> MSDSVILRSIKKFGEENDGFESDKSYNNDKKSRLQDEKKGDGVRVGFFQLFRFSSSTDIWLMFVGSLCAFLHGIAQPGVLLIFGTMTDVFIDYDVELQELQIPGKACVNNTIVWTNSSLNQNMTNGTRCGLLNIESEMIKFASYYAGIAVAVLITGYIQICFWVIAAARQIQKMRKFYFRRIMRMEIGWFDCNSVGELNTRFSDDINKINDAIADQMALFIQRMTSTICGFLLGFFRGWKLTLVIISVSPLIGIGAATIGLSVSKFTDYELKAYAKAGVVADEVISSMRTVAAFGGEKREVERYEKNLVFAQRWGIRKGIVMGFFTGFVWCLIFLCYALAFWYGSTLVLDEGEYTPGTLVQIFLSVIVGALNLGNASPCLEAFATGRAAATSIFETIDRKPIIDCMSEDGYKLDRIKGEIEFHNVTFHYPSRPEVKILNDLNMVIKPGEMTALVGPSGAGKSTALQLIQRFYDPCEGMVTVDGHDIRSLNIQWLRDQIGIVEQEPVLFSTTIAENIRYGREDATMEDIVQAAKEANAYNFIMDLPQQFDTLVGEGGGQMSGGQKQRVAIARALIRNPKILLLDMATSALDNESEAMVQEVLSKIQHGHTIISVAHRLSTVRAADTIIGFEHGTAVERGTHEELLERKGVYFTLVTLQSQGNQALNEEDIKDATEDDMLARTFSRGSYQDSLRASIRQRSKSQLSYLVHEPPLAVVDHKSTYEEDRKDKDIPVQEEVEPAPVRRILKFSAPEWPYMLVGSVGAAVNGTVTPLYAFLFSQILGTFSIPDKEEQRSQINGVCLLFVAMGCVSLFTQFLQGYAFAKSGELLTKRLRKFGFRAMLGQDIAWFDDLRNSPGALTTRLATDASQVQGAAGSQIGMIVNSFTNVTVAMIIAFSFSWKLSLVILCFFPFLALSGATQTRMLTGFASRDKQALEMVGQITNEALSNIRTVAGIGKERRFIEALETELEKPFKTAIQKANIYGFCFAFAQCIMFIANSASYRYGGYLISNEGLHFSYVFRVISAVVLSATALGRAFSYTPSYAKAKISAARFFQLLDRQPPISVYNTAGEKWDNFQGKIDFVDCKFTYPSRPDSQVLNGLSVSISPGQTLAFVGSSGCGKSTSIQLLERFYDPDQGKVMIDGHDSKKVNVQFLRSNIGIVSQEPVLFACSIMDNIKYGDNTKEIPMERVIAAAKQAQLHDFVMSLPEKYETNVGSQGSQLSRGEKQRIAIARAIVRDPKILLLDQATSALDTESEKTVQVALDKAREGRTCIVIAHRLSTIQNADIIAVMAQGVVIEKGTHEELMAQKGAYYKLVTTGSPIS

BSEP (ABCB11) is an ATP-binding cassette transporter that is expressed in hepatocytes and extrudes bile salts into the canaliculi of the liver. BSEP dysfunction, caused by mutations or induced by drugs, is frequently associated with severe cholestatic liver disease. BSEP has two transmembrane domains (TMDs), each composed of six TM helices, and two nucleotide-binding domains (NBDs). The NBDs of BSEP are predicted to form one functional nucleotide-binding site (NBS2, consisting of Walker-A and Walker-B motifs of NBD2 and the signature motif of NBD1), and one degenerate nucleotide-binding site (NBS1, consisting of Walker-A and Walker-B motifs of NBD1 and the signature motif of NBD2).

Human wild-type BSEP and a variant in which the catalytic glutamate of NBS2 was replaced by a glutamine (E1244Q) were expressed in HEK293 stable cell lines and purified in detergent. No ATPase activity was observed for BSEPE1244Q in detergent or in proteoliposomes, even at elevated concentrations of ATP and TC. To capture BSEP in a nucleotide-bound state, nanodisc-reconstituted BSEPE1244Q in the presence of TC and ATP was prepared for cryo-EM studies. Approximately 60% of the particles adopted a closed state and yielded a cryo-EM density map at a resolution of 3.0 Å. We observed tightly packed TMDs and NBDs in a closed conformation. No substrate binding cavity is present between the TMDs, suggesting that this conformation may represent a state of post-substrate release. We observed two distinct EM densities in the two NBSs, each corresponding to an ATP molecule, which is consistent with the characteristic architecture of other ABC transporters. ATP binding is mediated by the Walker-A motif interacting with the phosphate groups and the A-loop interacting with the purine ring of ATP through π–π stacking. We also observed clear densities for bound Mg2+ ions in the two NBSs, which are coordinated by the beta and gamma phosphates of ATP, the glutamine residues of the Q-loop (Q503 and Q1161), the serine residues of the Walker-A motifs (S462 and S1120), the aspartate residues of the Walker-B motifs (D583 and D1243), and water molecules. BSEPE1244Q represents a state prior to ATP hydrolysis, whereas vanadate-trapped BSEP represents a state immediately after ATP hydrolysis.> SVRVMQLTLGNSTITTQEAANSVVAYGRWPEYIKDSEANPVDQPTEPDVAACRFYTLDTVTWRKESRGWWWKLPDALKDMGLFGQNMFYHYLGRAGYTVHVQCNASKFHQGALGVFAVPEMCLAGDSTTHMFTKYENANPGEKGGEFKGSFTLDTNATNPARNFCPVDYLFGSGVLAGNAFVYPHQIINLRTNNCATLVLPYVNSLSIDSMTKHNNWGIAILPLAPLDFATESSTEIPITLTIAPMCCEFNGLR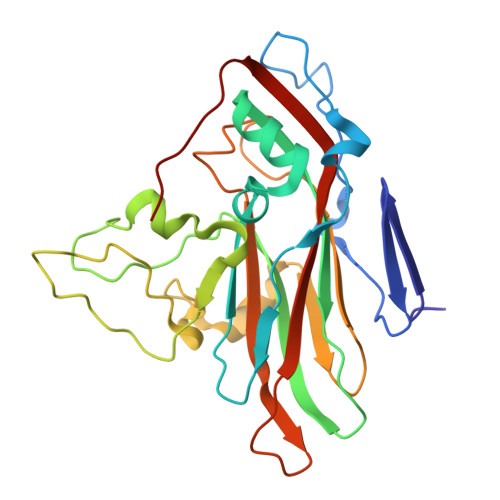NITVPRTQ Peptidyl-prolyl isomerases (PPIases) catalyze intrinsically slow and often rate-limiting isomerization of prolyl-peptide bonds in unfolded or partially folded proteins, thereby speeding up the folding process and preventing misfolding. An example of such a protein is SlyD (Sensitive to Lysis D), which consists of an FKBP type PPIase domain and a chaperone domain, called IF (insert-in-flap) domain, that has been shown to exhibit chaperone activity. Each of these domains contains one binding site for unfolded proteins or peptides. Often, FKBPs are linked to an additional chaperone domain that can increase their PPIase activity by up to 200-fold.

The activity profile for peptides with alanine residues in different positions confirms the importance of W4 and F13 to the enzymatic activity in the full-length context, while removing the methionine side chain in the M8A peptide increases the enzymatic activity. Although most of the protein–peptide complexes did not crystallize or yielded crystals of poor diffraction quality, we succeeded in structure determination for four complexes of SlyDWT with bound substrates: psWT, W4A, W4K, and M8A. In all structures, the peptide substrates are bound in the PPIase binding pocket with the proline residue in cis conformation, coordinated by the previously observed protein–peptide polar interactions, namely N35-L9, I37-L9, Y63-F11, H119-F11 and Y92-F13. On the other hand, the conformational flexibility of the residue i − 6 is also reflected in our crystal structures.While residue W4 of the original S2 peptide forms a polar interaction with the SlyD residue E60, orienting the N-terminus of the peptide outside of the binding pocket, mutant peptide residues A4 and K4 do not form this interaction and as a result, the peptide N-terminus bends towards the SlyD linker region. Taken together, while different side chains at position 4 assume distinct conformations in each substrate variant, these conformations proof to be unspecific when compared to the structure of other variants. This resembles encounter complexes where initial contacts are unspecific and contribute to the association reaction, but not to the dissociation step where they are replaced by specific contacts. When both binding sites are fully occupied, the two domains restrict access to the PPIase domain binding site in the tight conformation. Here, the release of the substrate from the FKBP binding site is likely hindered.

> MKVGQDKVVTIRYTLQVEGEVLDQGELSYLHGHRNLIPGLEEALEGREEGEAFQAHVPAEKAYGPHDPEGVQVVPLSAFPEDAEVVPGAQFYAQDMEGNPMPLTVVAVEGEEVTVDFNHPLAGKDLDFQVEVVKVREATPEELLHGHAHPSGHHHHHH;>[2x]TRYANAKMLPFAFGA>MRQFIISENTMQKTSFRNHQVKRFSSQRSTRRKPENQPTRVILFNKPYDVLPQFTDEAGRKTLKEFIPVQGVYAAGRLDRDSEGLLVLTNNGALQARLTQPGKRTGKIYYVQVEGIPTQDALEALRNGVTLNDGPTLPAGAELVDE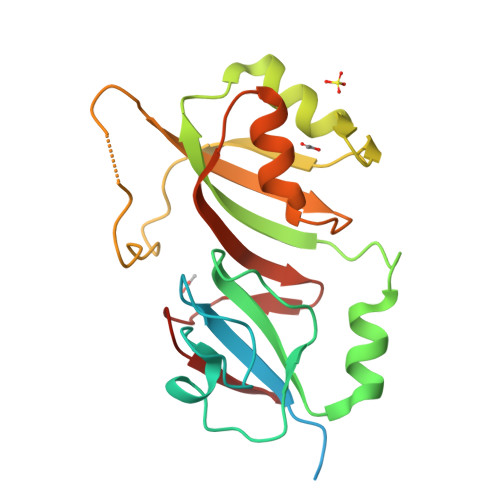PAWLWPRNPPIRERKSIPTSWLKITLYEGRNRQVRRMTAHVGFPTLRLIRYAMGDYSLDNLANGEWREVTD[2x]>GSHMAAGGDHGSPDSYRSPLASRYASPEMCFVFSDRYKFRTWRQLWLWLAEAEQTLGLPITDEQIREMKSNLENIDFKMAAEEEKRLRHDVMAHVHTFGHCCPKAAGIIHLGATSCYVGDNTDLIILRNALDLLLPKLARVISRLADFAKERASLPTLGFTHFQPAQLTTVGKRCCLWIQDLCMDLQNLKRVRDDLRFRGVKGTTGTQASFLQLFEGDDHKVEQLDKMVTEKAGFKRAFIITGQTYTRKVDIEVLSVLASLGASVHKICTDIRLLANLKEMEEPFEKQQIGSSAMPYKRNPMRSECCCSLARHLMTLVMDPLQTASVQWFERTLDDSANRRICLAEAFLTADTILNTLQNISEGLVVYPKVIERRIRQELPFMATENIIMAMVKAGGSRQDCHEKIRVLSQQAASVVKQEGGDNDLIERIQVDAYFSPIHSQLDHLLDPSSFTGRASQQVQRFLEEEVYPLLKPYESVMKVKAE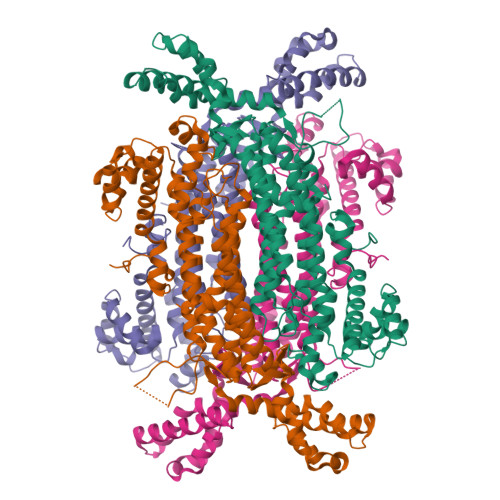LCL[4x]>[2x]LGLSITGLGVQYPPYSLGPDAIDILSKRYHPESPAMKKVLAINRYTGIDQRSSIGNPDHPLVNKPNPPTVKELHEVFMSDGVPLAV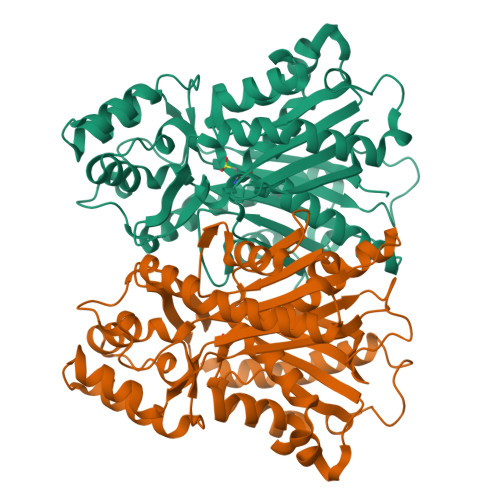EASRKAMAEARLVPAQITHMVSTTCTDSANPGYDHYVAKELGLSDRLEKVLLHGIGCSGGLAALRTAANLCLGHTARGKPARILVLALEVSTTMVRSELESIDALQETRIGIALFSDCASAVILSNGIGEAPGKPAIYDLLGWENRVIPDSEHDLGFDVDPMGWKVVLSPRVPVLAKASLQPTYADLLSSLQDQLPSSYQKPADFDWAMHPGGATILSGAESAMGLTPEHMRASYDRYINHGNSSSATIFSVLNRLREKDMDALAPGGKVKEYVVGCAFGPGINVEMCMLKRR> SSLIKKIEENERKDTLNTLQNMFPDMDPSLIEDVCIAKKS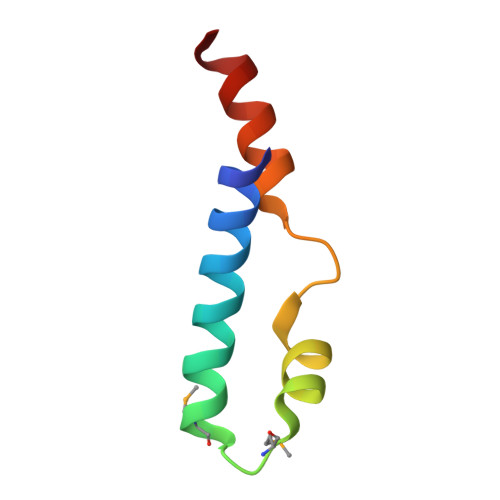RIEPCVDALLSLSE> CSCSSLMDKECVYFCHLDIIW;> PGGGLAPAEVPKGDRTAGSPPRTISPPPCQGPIEIKETFKYINTVVSCLVFVLGIIGNSTLLYIIYKNKCMRNGPNILIASLAL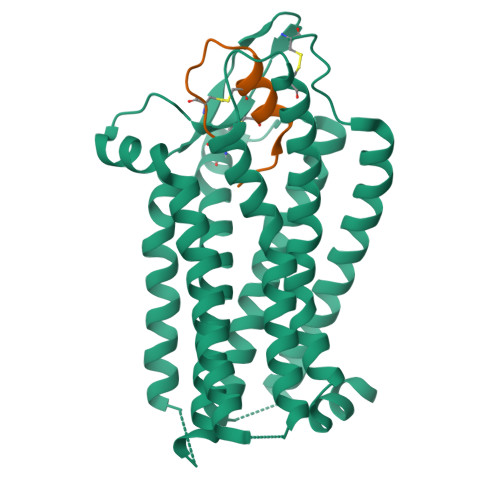GDLLHIVIDIPINVYKLLAEDWPFGAEMCKLVPFIQKASVGITVLSLCALSIDRYRAVASWSRIKGIGVPKWTAVEIVLIWVVSVVLAVPEAIGFDIITMDYKGSYLRICLLHPVQKTAFMQFYKTAKDWWLFSFYFCLPLAITAFFYTLMTCEMLRKKSGMQIALNDHLKQRREVAKTVFCLVLVFALCWLPLHLSRILKLTLYNQNDPNRCELLSFLLVLDYIGINMASLNSCINPIALYLVSKRFKNAFKSALCCWAQS> GVEEKKSLEILLKDDRLDTEKLCTFSQRFPLPSMYRALVWKVLLGILPPHHESHAKVMMYRKEQYLDVLHALKVVRFVSDATPQAEVYLRMYQLESGKLPRSPSFPLEPDDE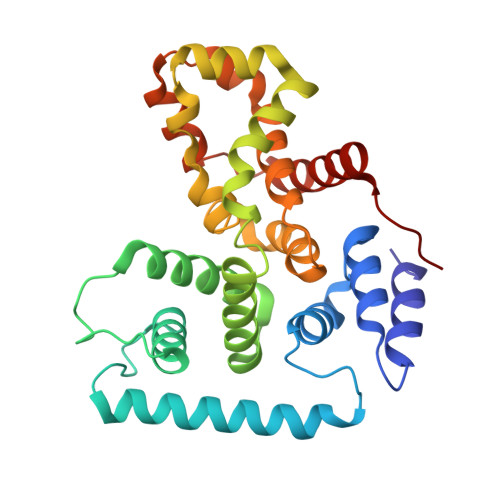VFLAIAKAMEEMVEDSVDCYWITRRFVNQLNTKYRDSLPQLPKAFEQYLNLEDGRLLTHLRMCSAAPKLPYDLWFKRCFAGCLPESSLQRVWDKVVSGSCKILVFVAVEILLTFKIKVMALNSAEKITKFLENIPQDSSDAIVSKAIDLWHKHCGTPVHSS> GKLTEGVNPGDLAPRIEFLGNDAKASFHNQLGRYTLLNFWAAYDAESRARNVQLANEVNKFGPDKIAMCSISMDEKESIFTETVKIDKL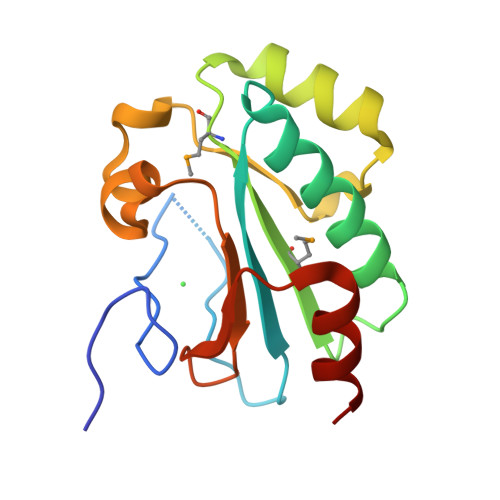DLSTQFHEGLGKESELYKKYDLRKGFKNFLINDEGVIIAANVTPEKLTEILKAI> GRKKIQISRILDQRNRQVTFTKRKFGLMKKAYELSVLCDCEIALIIFNSANRLFQYASTDMDRVLLKYTEYS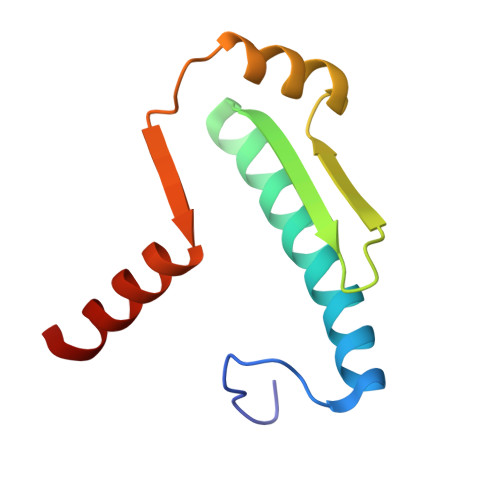EPHESRTNTDILETLKRRGIG> MSEKTTKGVQLLRGDPKKAIVRLSIPMMIGMSVQTLYNLADGIWVSGLGPESLAAVGLFFPVFMGIIALAAGLGVGTSSAIARRIGARDKE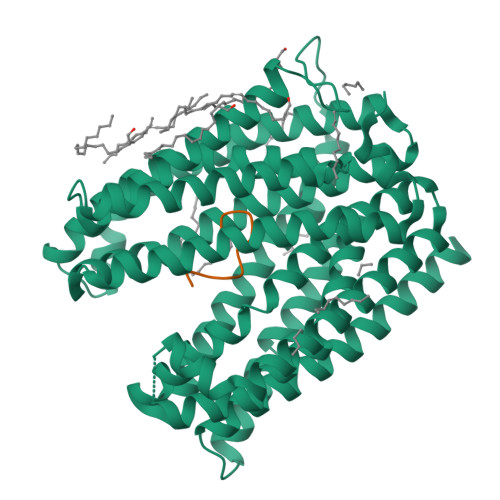GADNVAVHSLILSLILGVTITITMLPAIDSLFRSMGAKGEAVELAIEYARVLLAGAFIIVFNNVGNGILRGEGDANRAMLAMVLGSGLNIVLDPIFIYTLGFGVVGAAYATLLSMVVTSLFIAYWLFVKRDTYVDITLRDFSPSREILKDILRVGLPSSLSQLSMSIAMFFLNSVAITAGGENGVAVFTSAWRITMLGIVPILGMAAATTSVTGAAYGERNVEKLETAYLYAIKIAFMIELAVVAFIMLFAPQVAYLFTYSESAQVIKGDLISALRTLPVFLVLTPFGMMTSAMFQGIGEGEKSLILTIFRTLVMQVGFAYIFVHYTTLGLRGVWIGIVIGNMVAAIVGFLWGRMRISALKKTSATGGKR;> XFVYSAVCLYV> MRLFYAVFLPEEVRAALVEAQTKVRPFRGWKPVPPHQLHLTL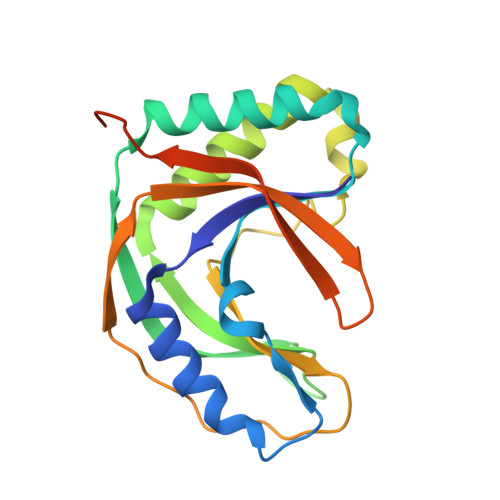LFLGERPEEELPDYLALGHRLARLEAPFRARLRGTGYFPNEGTPRVWFAKAEAEGFLRLAEGLRAGVEELLGEEAVRIPGWDKPFKPHITLARRKAPAPRVPPVLFGLEWPVEGFALVRSELKPKGPVYTVLEKFSLRGEHGREQAQGPGERPEGD(2R)-2-[[4-[[4-[(Z)-(2,4-dioxo-1,3-thiazolidin-5-ylidene)methyl]phenoxy]methyl]phenyl]sulfonylamino]pentanedioic acid | C22 H20 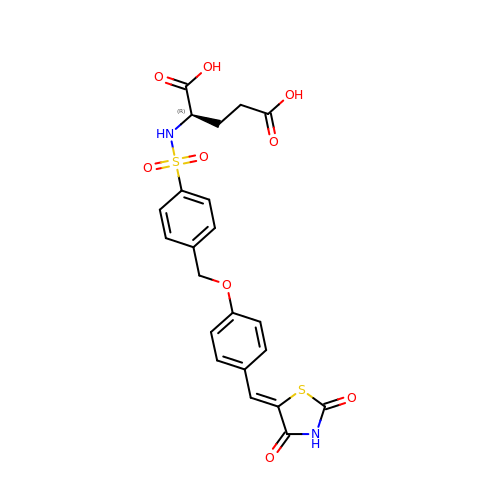N2 O9 S2 | BZCXCLVFYJNKLW-LVSMMTLPSA-N>MVVTRIAPSPTGDPHVGTAYIALFNYAWARRNGGRFIVRIEDTDRARYVPGAEERILAALKWLGLSYDEGPDVGGPHGPYRQSERLPLYQKYAEELLKRGWAYRAFETPEELEQIRKEKGGYDGRARNIPPEEAEERARRGEPHVIRLKVPRPGTTEVKDELRGVVVYDNQEIPDVVLLKSDGYPTYHLANVVDDHLMGVTDVIRAEEWLVSTPIHVLLYRAFGWEAPRFYHMPLLRNPDKTKISKRKSHTSLDWYKAEGFLPEALRNYLCLMGFSMPDGREIFTLEEFIQAFTWERVSLGGPVFDLEKLRWMNGKYIREVLS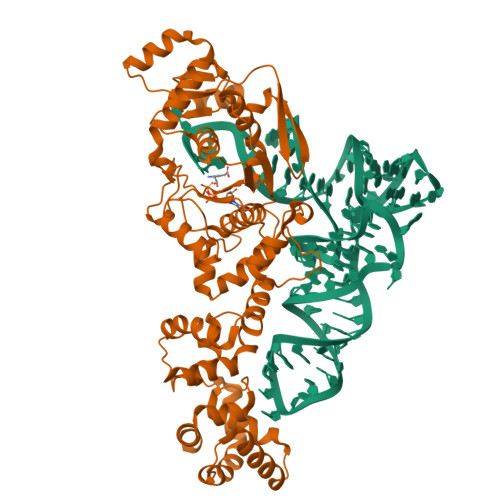LEEVAERVKPFLREAGLSWESEAYLRRAVELMRPRFDTLKEFPEKARYLFTEDYPVSEKAQRKLEEGLPLLKELYPRLRAQEEWTEAALEALLRGFAAEKGVKLGQVAQPLRAALTGSLETPGLFEILALLGKERALRRLERALA[2x]>[4x]GSMSEQSICQARAAVMVYDDANKKWVPAGGST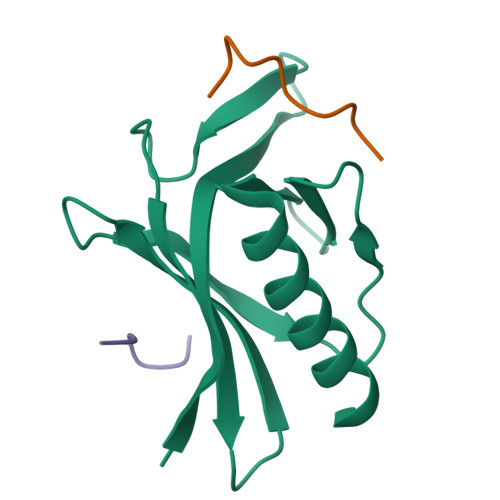GFSRVHIYHHTGNNTFRVVGRKIQDHQVVINCAIPKGLKYNQATQTFHQWRDARQVYGLNFGSKEDANVFASAMMHALEVL;>XWPPPPTEDELX[8x]> MGSSHHHHHHGSMYGVYRAMKLPIYLDYSATTPVDPRVAEKMMQFMTMDGTFGNPASRSHRFGWQAEEAVDIARNQIADLVGADPREIVFTSGATESDNLAIKGAANFYQKKGKHIITSKTEHKAVLDTCRQLEREGFEVTYLAPQRNGIIDLKELEAAMRDDTILVSIMHVNNEIGVVQDIAAIGEMCRARGIIYHVDATQSVGK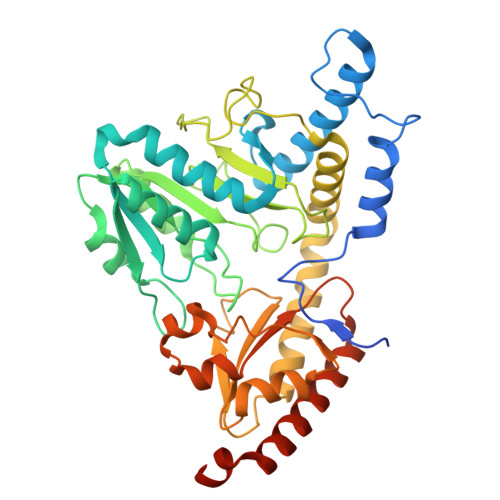LPIDLSQLKVDLMSFSGHKIYGPKGIGALYVRRKPRVRIEAQMHGGGHERGMRSGTLPVHQIVGMGEAYRIAKEEMATEMERLRGLRNRLWNGIKDIEEVYLNGDLEHGAPNILNVSFNYVEGESLIMALKDLAVSSGSACTSASLEPSYVLRALGLNDELAHSSIRFSLGRFTTEEEIDYTIELVRKSIGRLRDLSPLWEMYKQGVDLNSIEWAHH>[7x]KSCCRNTLARNCYNACRFTGGSQPT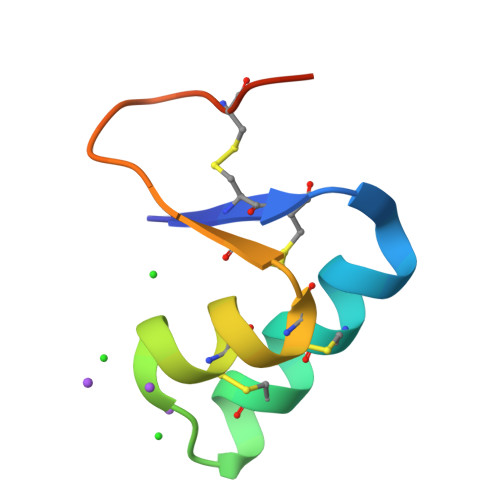CGILCDCIHVTTTTCPSSHPS> STGYQNILGQRNQNALNFDIQEDFETRLAKIKKDGGSGNDVEIFTYRIGKNGRSNSVSVKGTTLSYKDNKVKNIHLFAANKKEIPLDIPEDLVVSLKDTNRYYYYAGETGPAGQAGFKDNKQSTKAKIHTSSAWFLSESSINYNNSRIVPVGTLGSNVQDQGFGIVLPKLPDDFQQISSNEKPIAITDEMRGRYLTFAARGINSFGRVGKYQEGPQRIWVMGLPNRGMRSNLVLHTDADLALMRNSDNTISAIPADGVAHTNTVVANYAETKKNGVYGAVIPVINYKEPAINQTRQLIALNDSKIQFSNHDFNKGYTTSMLIGNRQQTGSLLTYKLDNSLNWTVSLEANGKIAIETVDNTNANNGGRQYANVVLDYTKDNSI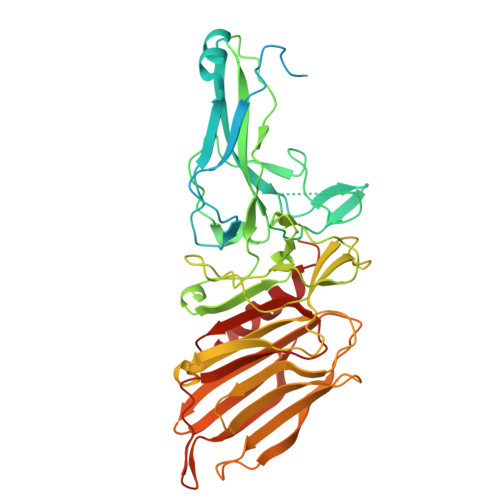QVRASVTNKILTLEVFVNGALVHTHELFMERNGVTHDIRKSQIIFGGKTFINEFAVYNKKLTDSEINILAEYFSDKYRAKA> GDRVADVIESSIGDSVSRALTHALPAPTGQN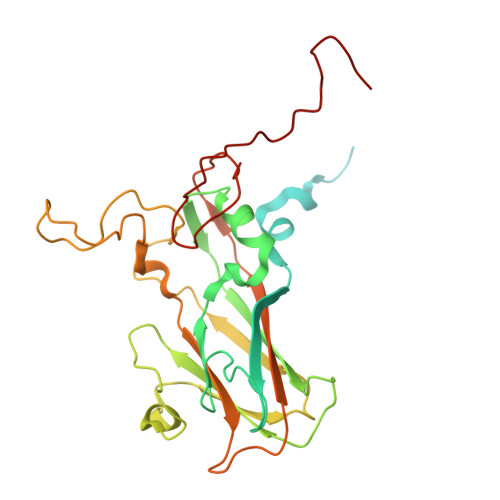TQVSSHRLDTGKVPALQAAEIGASSNASDESMIETRCVLNSHSTAETTLDSFFSRAGLVGEIDLPLEGTERKRARLTPNGYANWDIDITGYAQMRRKVELFTYMRFDAEFTFVACTPTGEVVPQLLQYMFVPPGAPKPDSRESLAWQTATNPSVFVKLSDPPAQVSVPFMSPASAYQWFYDGYPTFGEHKQEKDLEYGACPNNMMGTFSVRTVGTSKSKYPLVVRIYMRMKHVRAWIPRPMRNQNYLFKANPNYAGNSIKPTGASRTAITTL>[3x]MTAKDDYPSLSFQQDYVYIFSSDFQLSEELGVALINALSAKEIVPERLYVMLNDKTISFSFISKNKKSKNRVLSTEKKLNYKHISEYIVNEIEY;>[3x]MGSSHHHHHHSQDPVHFYETSYKYQAADSTYMHDVAINVSIKGNHFTSDIIIRELVKSENKNYYNVIGHGDIIQKNTHQYYLNFDNIDVYTGTNKANMKPYKEPTSISSLINKSNNIRVVYLSEEYVVVEFFFYDGQIITLHRY

In V. parahaemolyticus, the activation of T3SS2 by bile salts is regulated by two transmembrane ToxR-like transcription factors, VtrA (VPA1332) and VtrB (VPA1348). Furthermore, we demonstrate that the periplasmic domains of the transmembrane proteins, VtrA and VtrC, form a functional complex that binds bile salts to activate VtrA’s cytoplasmic DNA binding domain, which in turn induces T3SS2 via the downstream transcription factor VtrB. The structure of VtrA/VtrC periplasmic domains reveals an obligate heterodimer where VtrC recruits structural elements from VtrA to complete a β-barrel with a hydrophobic inner chamber that binds bile salts. Our biochemical data and the structural analysis demonstrated that the periplasmic domains of the inner membrane proteins VtrA and VtrC form a stable complex that functions as a receptor for bile salts.

We next purified the VtrA/VtrC heterodimer in the presence of the bile salt TDC and crystalized this complex and obtained its X-ray structure. The crystal structure was solved via molecular replacement by using our original VtrA/VtrC heterodimer as a search model, and refined to a resolution of 2.10 Å. The model reveals three VtrA/VtrC heterodimers in the asymmetric unit, each with clear electron density for one TDC molecule bound inside the β-barrel. A fourth TDC molecule mediated lattice contacts between VtrA chain A and its symmetry mate. Negative power deflections were observed throughout the titration of the bile salt TDC into the VtrA/VtrC solution. These results indicated that TDC binds to the VtrA/VtrC heterodimer in an exothermic manner, with a dissociation constant (KD) of 315.4 nM. Although the three heterodimers in the asymmetric unit are highly similar, average root mean squared deviations (RMSD) of 0.5 Å for VtrA and 0.6–1.5 Å for VtrC indicates that there are differences in the VtrC monomer. RSMD values of 0.4–0.5 Å for VtrA and 1.2–1.9 Å were obtained by superimposing each of the TDC-bound heterodimers to the apo structure (Figure 8—figure supplement 2B-–E), indicating that the overall fold is maintained but there are considerable changes in the VtrC monomer. The largest differences between the VtrA/VtrC-TDC and the apo heterodimers are in the VtrC disordered loop and Fα that follows it. In the VtrA/VtrC-TDC heterodimer, the disordered loop has been displaced by the TDC molecule and is now observable in two out of the three heterodimers in the crystallographic asymmetric unit. Remarkably, one of these residues (Ser123) now forms a hydrogen bond with the 12α-hydroxyl group of TDC. The main chain amide between F150 and Tyr151 (Hβ-Iβ loop) coordinates the 3α-hydroxyl group, which is present in all bile salts, suggesting that this interaction is important for specificity towards bile salts.Recently, two group A flavoprotein monooxygenases (FPMOs) (GrhO5 and GrhO6) and a flavoprotein oxidase (GrhO1) were shown to mediate the drastic remodeling of the 3 backbone and subsequent spiroketal pharmacophore formation. First, GrhO5 generates a ‐spiroketal moiety as part of the advanced intermediate dihydrolenticulone (4), which entails the rupture of three C−C bonds and a CO2 elimination step. The functional homolog RubL from rubromycin biosynthesis was shown to catalyze the same reaction sequence, pointing toward a universal strategy for spiroketal formation in the rubromycin family. In this work, the combined crystal structures of GrhO5 and RubL suggest three interconvertible catalytically relevant conformers, hereafter referred to as the “acceptor state” (FADox in OUT; accepts substrate, no reaction with NADPH), “reducible state” (FADox in OUT with bound substrate; reducible by NADPH) and the “catalytic state” (FADred in IN with bound substrate; reacts with O2 for hydroxylation).

To investigate the enzyme mechanism, GrhO5 crystals were soaked with 3. Gratifyingly, analysis of these crystals revealed clear electron density in the open, solvent‐exposed substrate‐binding site, consistent with the binding of 3 or 5 (possibly formed by X‐ray radiation induced reduction). In this conformation, the O1 and the O3 atoms were positioned in hydrogen‐bonding distance to the C4 carbonyl group and the N3 (only O1) of the isoalloxazine ring of FAD that retained the OUT conformation. This ternary complex (GrhO5, FAD, 3/5) represents the reducible state, in which the substrate is tightly coordinated by a cluster of basic amino acid side chains comprising H217, R79, and R366 that are in hydrogen‐bonding distance to O8/O10, O4/O5/O8/O9, and O4/O8 of 3/5, respectively. Interestingly, while the FAD conformation and active site residues were not affected by 3/5 binding, a distinct rotation of the conserved W281 side chain was observed that now adopts an intermediate position (with respect to its final position in the catalytic state, vide infra), while retaining the aromatic sandwich π‐π stacking with FAD. This is different from the type I members RebC and PieE, for which substrate soaking of the protein crystals induced the movement of the FAD cofactor to “IN” alongside the rotation of several amino acid side chains. Importantly, the novel snapshot of the GrhO5 reducible state shows that substrate binding first triggers a distinctive side chain motion of the corresponding W281 that enables the reaction with NADPH, while retaining the sandwich π‐π stacking interaction. Evidently, movement to IN did not occur in the soaked GrhO5 crystals, presumably because FAD unlocking also requires reduction to antiaromatic FADred in order to disrupt the sandwich π‐π stacking interaction with the flipped W281 side chain (consistent with the previously reported movement of artificially reduced FAD to IN in RebC crystals).

> MSSSGTRVLIVGGSLVGLSTAVFLAHHDVPVTLVERHPGTSIHPRAVGYYPRTAELLATVGVEAPAKAAASGFEKHRTRAGVESLAGEVLFSKEELEGGDELADLTPSSLLLLPQDRLEPILRARAEELGAELRFGAELRSFTQDADGVSAVVRDADGGESVVRADYLVAADGPRSTVREALGIGREGRGVLSRHVSIAFGADFAAVLGERRYSVVHVQNDRVTGILVHDDTLTEGTLIVGYDPEKGEGLDDFTDARCAELVSAAIGSDDVAVTIRSRFPWDMAELVADAFVSDRVLVAGDAAHQIPPTGGYGANTGIADAFNLSWKLAHVLAGTAGRALLDTYDEERRPVGLYTARQGSLQLAVRSRTATEEQREAAHDAMRVTMGQAYPSGAFVADAGADPLPLTSDPRTLRGEPGTRAPYVVLERDGAPLSTLDLFGDGFVLLVGADGGSWAEAAGEAAAGLGVGIAFHRVAPDAGEGRPVDVHGRWAEAYGVGAAGAVLVRPDGIVAWRSRDGMPGGAGGRALTAALRTVLAR> KKVIIAGNGPSLKEIDYSRLPNDFDVFRCNQFYFEDKYYLGKKCKAVFYAPSLFFEQYYTLKHLIQNQEYETELIMCSNYNQAHLENENFVKTFYDYFPDAHLGYDFFKQ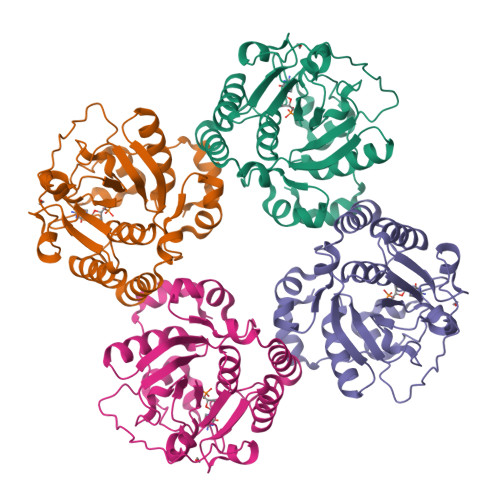LKDFNAYFKFHEIYFNQRITSGVYMCAVAIALGYKEIYLSGIDFYQNGSSYAFDTKQKNLLKLAPNFKNDNSHYIGHSKNTDIKALEFLEKTYKIKLYCLCPNSLLANFIGLAPNLNSNFIIQEKNNYTKDILIPSSEAYGKFSKNIN> MTRYYCEYCHSYLTHDTLSVRKSHLVGKNHLRITADYYRNKARDIINKHNHKRRHIGKRGRKERENSSQNETLKVTCLSNKEKRHIMHVKKMNQKELAQTSIDTLKLLYDGSPGYSKVFVDANRFDIGDLVKASKLPQRANEKSAHHSFKQTSRSRDETCESNPFPRLNNPKKLEPPKILSQWSNTIPKTSIFY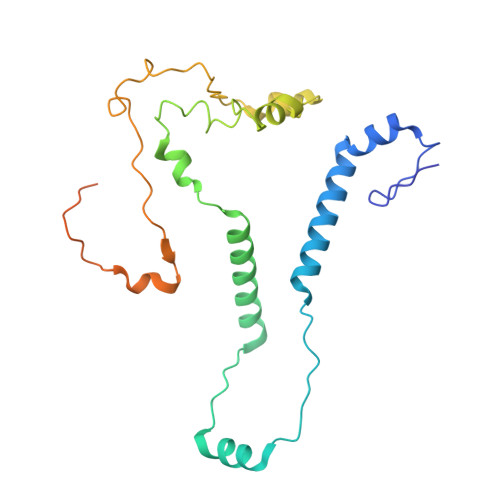SVDILQTTIKESKKRMHSDGIRKPSSANGYKRRRYGN> GCGUUGG;> 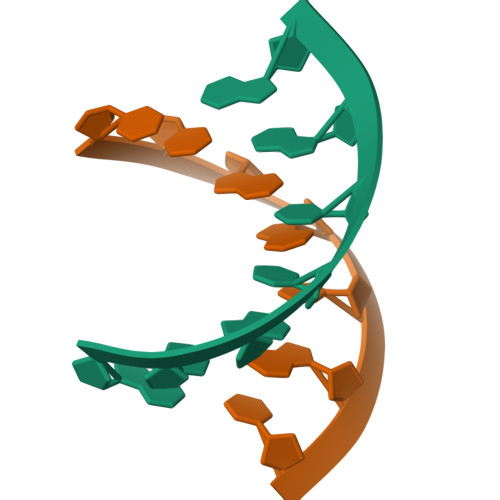CCAACGC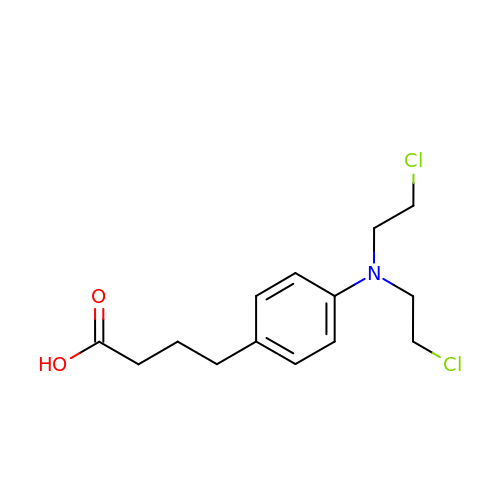CHLORAMBUCIL | C14 H19 Cl2 N O2 | JCKYGMPEJWAADB-UHFFFAOYSA-N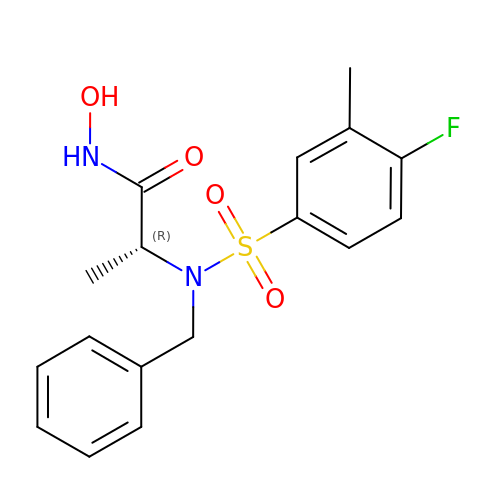N~2~-benzyl-N~2~-[(4-fluoro-3-methylphenyl)sulfonyl]-N-hydroxy-D-alaninamide | C17 H19 F N2 O4 S | ZVJSGLFNUKONDD-CYBMUJFWSA-N(2E)-N-hydroxy-3-{4-[(E)-(1,3,5-trimethyl-1H-pyrazol-4-yl)diazenyl]phenyl}prop-2-enamide | C15 H17 N5 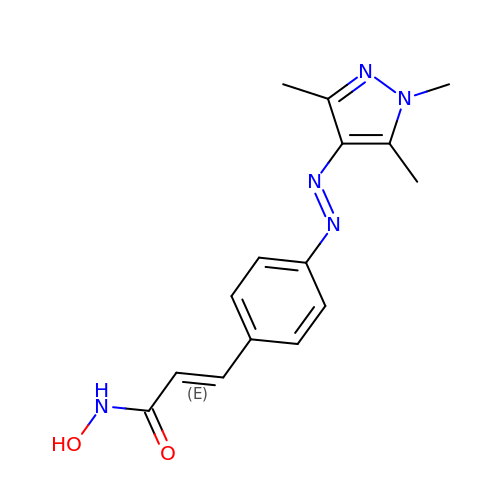O2 | GGZOJTXQALEQJU-OUWLFTCQSA-N>NMVHPNVICDGCNGPVVGTRYKCSVCPDYDLCSVCEGKGLHRGHTKLAFPSPF[4x];>[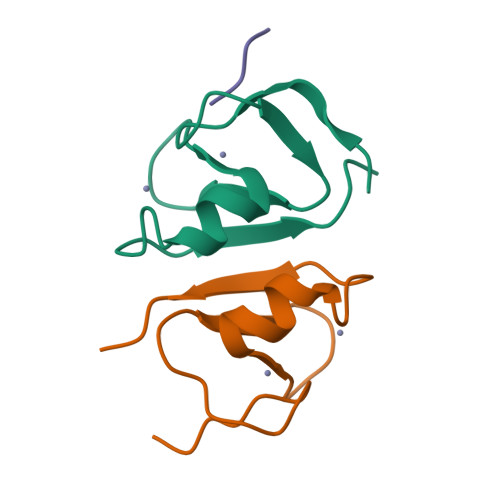2x]RIVPA> GSDLPAGWMRVQDTSGTYYWHIPTGTTQWEPPGRASPS;> PPPPPP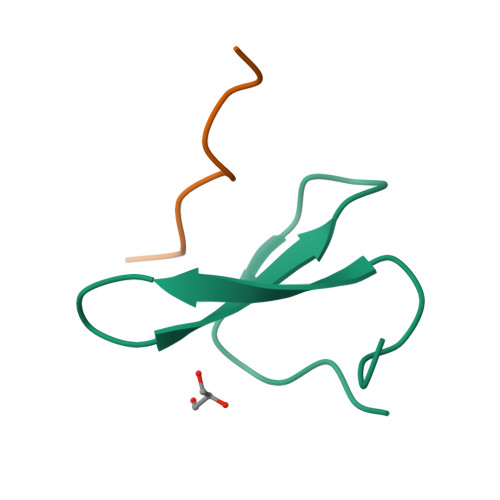PPPL Amplification of piRNA in the ping-pong cycle requires assembly of a tertiary complex scaffolded by Krimper, which simultaneously binds the N-terminal regions of Aub and Ago3. To promote generation of new piRNA, Krimper uses its two Tudor domains to bind Aub and Ago3 in opposite modification and piRNA-loading states. In addition to its self-interacting N-terminal region, Krimper contains two extended Tudor domains: eTud1(272-512) and eTud2 (562-746). Overall, our results reveal that the two Tudor domains of Krimper have distinct architectures that are responsible for the differential binding of two PIWI proteins.

Unlike eTud2, Krimper (eTud1) has an unusual binding specificity towards the unmethylated Ago3 sequence containing the (G/A)R motif. To elucidate the interaction between eTud1 and Ago3 we solved the crystal structure of eTud1 in both apo and peptide bound forms. However, the Ago3 peptide displaces the “latch helix” and adopts an α-helical structure to bind in the same cleft between the Tudor and SN-like subdomains, but with reverse directionality compared to the “latch helix”. The Ago3 peptide binds both a hydrophilic concave and a hydrophobic concave region in the cleft between the Tudor and SN-like subdomains of eTud1. However, instead of a conserved aromatic cage that interacts with sDMA in other canonical Tudor domains including eTud2, the binding of unmethylated Arg70 of Ago3 in eTud1 is provided by a mostly hydrophilic pocket composed of three non-aromatic amino acids (Asp373, Thr380, and Leu397). Arg70 forms hydrogen bonds with Asp373 and Glu402 in eTud1, supplemented by a cation-π interaction with Phe400. Notably, the side chain of Phe400 is rotated by 90° to form a stronger cation-π interaction with Arg70 when compared with the structure in the apostate. Adjacent to the hydrophilic concave region there exists a hydrophobic concave region formed by Phe400, Trp339, and Tyr446. The Ago3 peptide forms a hydrophobic contact with the hydrophobic concave region utilizing Leu73 and Leu77 that strengthens its interactions. Thus, eTud1 specifically recognizes unmodified R(A/G) motif in Ago3 using a unique hydrophilic concave and a hydrophobic concave region in the interface between the Tudor and SN-like subdomains.

>SASIEKVNKLPKSPRNRFLLPPKGGTETTRRDIYNQILKDMAAFPENTIVTAVLASVDVTDNCAYVAKWDESSDRIKKVLQRQLPLQELDQLPDYGDIFAVLDSINNIITRITINSSSAGGGYDAYLIDFGEHIHFDGNETIFKLPDDIKRLPAQAIRCDLINCDIANMHCFVNTYIKIRVHENNNSTLVAEPVIDRLSRPTKTNTTKYPAGITEDDMAMLNEIDESTSDPLKAVLGFRPKD[5x];>[4x]NISVGRGRARLIDTLK A tetratricopeptide repeat (TPR) motif containing mitochondrial outer membrane protein, mitochondrial fission protein 1 (Fis1), mediates mitochondrial fission by recruiting large cytosolic GTPase, Drp1, to the mitochondrial outer membrane. The cytosolic domain of Fis1 is composed of 6 tight α-helices with two anti-parallel TPR motifs forming a concave hydrophobic surface. Fis1 interaction with Drp1 occurs during cellular stress, but not under physiological conditions, suggesting that cellular signals during stress activate Fis1. Human Fis1 protein contains a single cysteine, Cys41, in the entire protein.

To explore this possibility further, we crystallized and determined the X-ray structures of the WT and three phosphorylation mimic-mutants of Fis1: Thr34Asp Fis1, Thr34Glu Fis1 and Tyr38Glu Fis1. Each of these mutants was previously shown to be sufficient to increase Drp1 recruitment to mitochondria and subsequent mitochondrial fission in cell-based studies. Consistently, we observed that the first 30 residues including the α1 helix were missing from the structure providing strong evidence that the α1 helix undergoes significant conformational change and is potentially disordered in the phosphorylated forms, whereas it was intact in the WT. We crystallized the phosphorylation-mimic mutants, Thr34Asp, Thr34Glu and Tyr38Glu Fis1, and we observed that in all the cases, these mutants crystallized as covalent dimers mediated by Cys41 disulfide bridge between two Fis1 protomers. As Thr34Asp, Thr34Glu and Tyr38Glu Fis1 have a greater propensity for a conformationally altered N-terminus and hence have more exposed Cys41, they crystallized as covalent dimers. Upon closer examination of the crystal structures, we observed that the concave hydrophobic surface in the covalent dimers of all the phosphorylation-mimic mutants was exposed. Our crystal structure not only shows the absence of α1 helix but also shows that there is no space for structured α1 helix in the covalent dimer as this space is occupied by α2 helix of another monomer. Here we showed that Cys41 is also oxidizable and mediates Fis1 covalent dimerization through disulfide linkage. This oxidation-induced Fis1 dimerization was obvious in the crystal structures of Thr34Asp, Thr34Glu and Tyr38Glu Fis1, where we saw a clear electron density for the disulfide linkage. When we modeled the structure of Fis1 WT dimer using the Thr34Asp Fis1 covalent dimer with modeled the missing unstructured first 30 residues, the Fis1 covalent WT dimer perfectly fitted the SAXS curve for WT Fis1 dimer.

> MEAVLNELVSVEDLLKFEKKFQSEKAAGSVSKSDQFEYAWCLVRSKYNDDIRKGIVLLEELLPKGSKEEQRDYVFYLAVGNYRLKEYEKALKYVRGLLQTEPQNNQAKELERLIDKAMKKDGLLEVLFQ>[2x]MTGDHIKVIYFNGRGRAESILMTLVAAGVNYEDERISFQDWPKIKPTIPG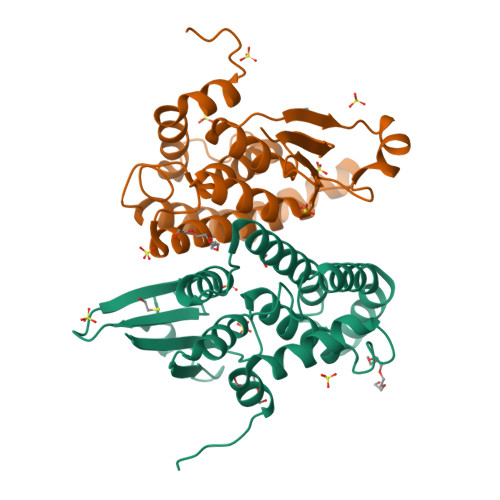GRLPAVKITDNHGHVKWMVESLAIARYMAKKHHMMGGTEEEYYNVEKLIGQAEDLEHEYYKTLMKPEEEKQKIIKEILNGKVPVLLDIICESLKASTGKLAVGDKVTLADLVLIAVIDHVTDLDKEFLTGKYPEIHKHRENLLASSPRLAKYLSDRAATPF> MPFPFGKSHKSPADIVKNLKESMAVLEKQDISDKKAEKATEEVSKNLVAMKEILYGTNEKEPQTEAVAQLAQELYNSGLLSTLVADLQLIDFEGKKDVAQIFNNILRRQIGTRTPTVEYICTQQNILFMLLKGYESPEIALNCG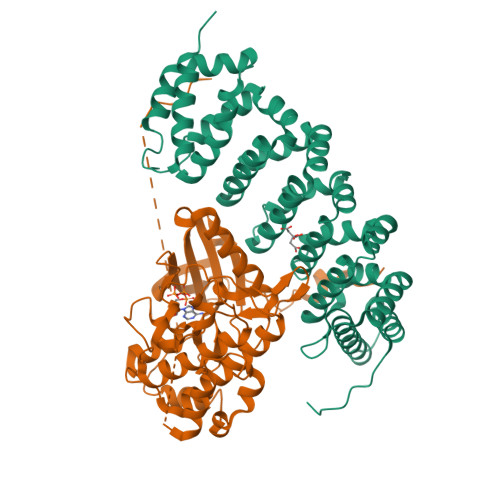IMLRECIRHEPLAKIILWSEQFYDFFRYVEMSTFDIASDAFATFKDLLTRHKLLSAEFLEQHYDRFFSEYEKLLHSENYVTKRQSLKLLGELLLDRHNFTIMTKYISKPENLKLMMNLLRDKSRNIQFEAFHVFKVFVANPNKTQPILDILLKNQAKLIEFLSKFQNDRTEDEQFNDEKTYLVKQIRDLKRPAQQEA;> MAHHHHHHMENLYFQGMSSFLPEGGCYELLTVIGKGFEDLMTVNLARYKPTGEYVTVRRINLEACSNEMVTFLQGELHVSKLFNHPNIVPYRATFIADNELWVVTSFMAYGSAKDLICTHFMDGMNELAIAYILQGVLKALDYIHHMGYVHRSVKASHILISVDGKVYLSGLRSNLSMISHGQRQRVVHDFPKYSVKVLPWLSPEVLQQNLQGYDAKSDIYSVGITACELANGHVPFKDMPATQMLLEKLNGTVPCLLDTSTIPAEELTMSPSRSVANSGLSDSLTTSTPRPSNGDSPSHPYHRTFSPHFHHFVEQCLQRNPDARPSASTLLNHSFFKQIKRRASEALPELLRPVTPITNFEGSQSQDHSGIFGLVTNLEELEVDDWEF> MAMLTKFESRSSRAKGVAFHPTQPWILTSLHNGRIQLWDYRMGTLLDRFDGHDGPVRGIAFHPTQPIFVSGGDDYKVNVWNYKSRKLLFSLCGHMDYVRVCTFHHEYPWILSCSDDQTIRIWNWQSRNCIAILTGHSHYVMCAAFHPSEDLIVSASLDQTVRVWDISGLRMKNAAPVSMSKEDQKAQAHNSISNDLFGS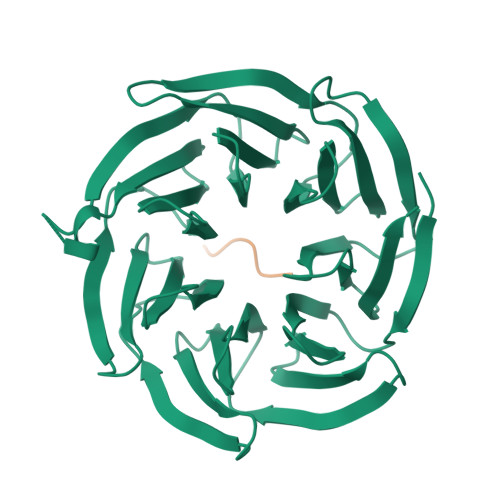ADAIVKFVLEGHDRGVNWCAFHPTLPLILSAGDDRLVKLWRMTASKAWEVDTCRGHFNNVSCCLFHPHQELILSASEDKTIRVWDLNRRTAVQTFRRANDRFWFITVHPKLNLFAAAHDSGVMVFKLE;> LKTKLL3-[[2-(trifluoromethyl)phenyl]methylamino]pyrazine-2-carboxamide | C13 H11 F3 N4 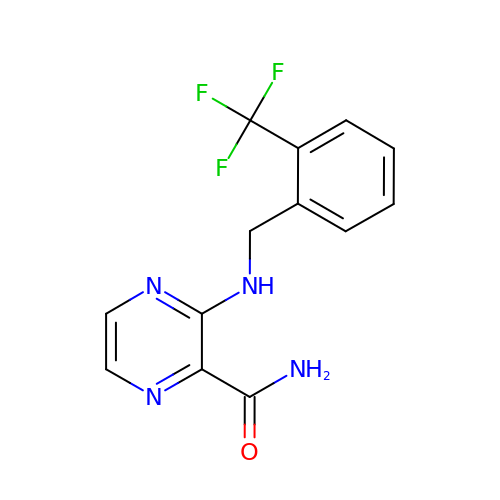O | RMLXGTUJQFYZEY-UHFFFAOYSA-N>TIVTDNSTGNHDGYDYEFWKDSGGSGTMILNSGGTFSASW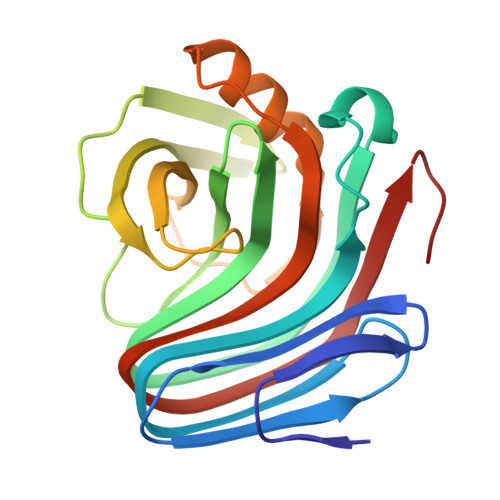NNVNNILFRKGKKFNETQTHQQVGNMSINYGANFQPNGNAYLCVYGWTVDPLVEYYIVDSWGNWRPPGATPKGTITVDGGTYDIYETLRVNQPSIKGIATFKQYWSVRRSKRTSGTISVSNHFRAWENLGMNMGKMYEVALTVEGYQSSGSANVYSNTLRINGNPL[2x]> MLRAKVRRIALANQKGGVGKTTTAINLAAYLARLGKRVLLVDLDPQGNATSGLGVRAERGVYHLLQGEPLEGLVHPVDGFHLLPATPDLVGATVELAGAPT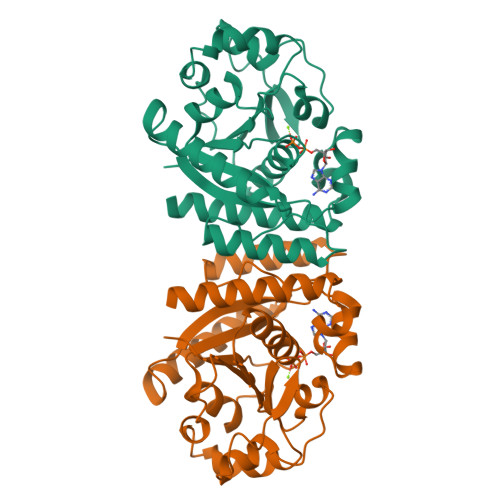ALREALRDEGYDLVLLDAPPSLSPLTLNALAAAEGVVVPVQAEYYALEGVAGLLATLEEVRAGLNPRLRLLGILVTMYDGRTLLAQQVEAQLRAHFGEKVFWTVIPRNVRLAEAPSFGKTIAQHAPTSPGAHAYRRLAEEVMARVQEAGSHHHHHH> MNLLETRRSLLEEMEIIENAIAERIQRNPELYYHYIQESSKVFPDTKLPRSSLIAENKIYKFKKVKRKRKQIILQQHEINIFLRDYQEKQQTFNKINRPEETQEDDKDLPNFERKLQQLEKELKNEDENFELDINSKKDKYALFSSSSDPSRRTNILSDRARDLDLNEIFTRDEQYGEYMELEQFHSLWLNVIKRGDCSLLQFLDILELFLDDEKYLLTPPMDRKNDRYMAFLLKLSKYVETFFFKSYALLDAAAVENLIKSDFEHSYCRGSLRSEAKGIYCPFCSRWFKTSSVFESHLVGKIHKKNESKRRNFVYSEYKLHRYLKYLNDEFSRTRSFVERKLAFTANERMAEMDILTQKYEAPAYDSTEKEGAE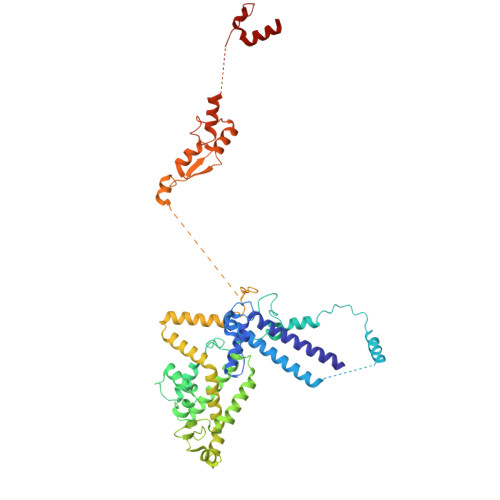QVDGEQRDGQLQEEHLSGKSFDMPLGPDGLPMPYWLYKLHGLDREYRCEICSNKVYNGRRTFERHFNEERHIYHLRCLGIEPSSVFKGITKIKEAQELWKNMQGQSQLTSIAAVPPKPNPSQLKVPTELELEEEDEEGNVMSKKVYDELKKQGLV> GPHMHKVKLAAITCELPARSYENDDPVFAAVPDLSESWWQFWGVNRRGYFDPRNGENEFSLVVRAAERLLRSSDTAPDSVDMLICSASSPIMTDAGDVLPDLRGRLYPRMANVLSKQLGLSRALPLDSQMESASFLLNLRLAASMIRQGKAEKVLVVCSEYISNLLDFTSRTSTLFADGCAVALLTRGDDDSCDLLASAEHSDATFYEVATGRWRLPENPTGEAKPRLYFSLFSDGQNKMASFVPTNVPIAMRRALEKAGLGSDDIDYFVFHQPAPFLVKAWAEGIGARPEQYQLTMGDTGVMISVSIPYTLMTGLREGKIRPGDRIVMAGAATGWGFAAQVWQLGEVL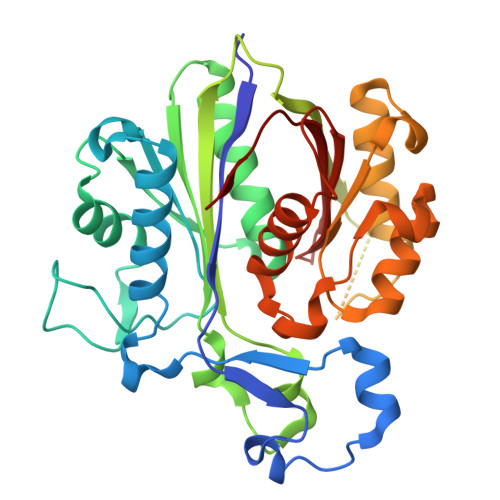VC>TGCVLNKLFQLPTPPLSRHQLKRLEEHRYQSAGRSLLEPLMQGYWEWLVRRVPSWIAPNLITIIGLSINICTTILLVFYCPTATEQAPLWAYIACACGLFIYQSLDAIDGKQARRTNSSSPLGELFDHGCDSLSTVFVVLGTCIAVQLGTNPDWMFFCCFAGTFMFYCAHWQTYVSGTLRFGIIDVTEVQIFIIIMHLLAVIGGPPFWQSMIPVLNIQMKIFPALCTVAGTIFSCTNYFRVIFTGGVGKNGSTIAGTSVLSPFLHIGSVITLAAMIYKKSAVQLFEKHPCLYILTFGFVSAKITNKLVVAHMTKSEMHLHDTAFIGPALLFLDQYFNSFIDEYIVLWIALVFSFFDLIRYCVSVCNQIASHLHIHVFRIK[2x]

Choline/ethanolamine phosphotransferase 1 (CEPT1) catalyzes the last step of the biosynthesis of PC and PE in the Kennedy pathway by transferring the substituted phosphate group from CDP-choline/ethanolamine to diacylglycerol. CPT1, CEPT1 and EPT1 belong to the CDP-alcohol phosphotransferase (CDP-AP) family, whose members share a common property of catalyzing the transfer of a substituted phosphate group from a CDP-linked donor to an acceptor alcohol. CEPT1 is a dimer with 10 transmembrane segments (TMs) in each protomer. TMs 1-6 constitute a conserved catalytic domain with an interior hydrophobic chamber accommodating a PC-like density.

We, therefore, incubated purified enzyme with 10 mM CDP-choline and then prepared cryo-samples. Eventually, we obtained a 3D map at 3.8 Å resolution. The overall structure is almost identical to our first structure with r.m.s.d. of 0.4 Å over 368 Cα atoms. However, the lipid-shaped density disappeared in the hydrophobic chamber, and a new density arose in the catalytic cavity. The CDP-choline molecule matches well with the new density. CDP-choline is primarily coordinated by the CDP-binding motif. The cytidine group is sandwiched between TM2 and TM3 and potentially forms hydrogen bonds with Asn86 and Glu151. Minor shifts of TMs 2/3 were observed to leave efficient space to accommodate the cytidine moiety. The pyrophosphate moiety is stabilized by the two metal ions that are coordinated by four conserved aspartate residues from the CDP-binding motif. The trimethylammonium group of choline may also be stabilized by Glu65, similar to what we observed in the PC coordination.>[2x]MGHHHHHHMGQLRLAVITTAKYFIPRLIGPFCQRYPGINVSLKVTNHEGLI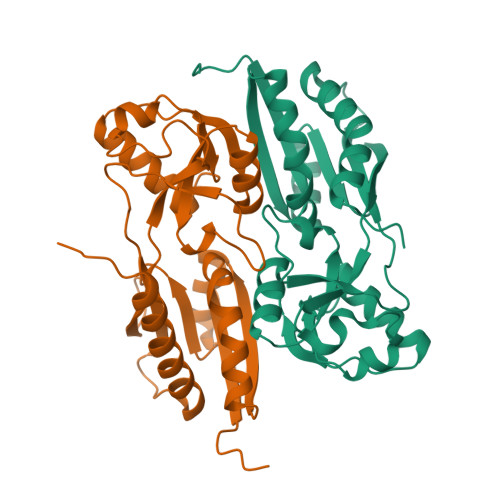NRINDNLDDLYVLSRPPSGFDITVQPFLDNPLVVVGPASHPLANQRGISLERLAQEPFILRERGSGTREATEQLFAAHNLNLNVKLDLGSNEAIKQAILGGLGLAVLSYHTLTSAGATPELKMFEVEGFPIHRQWHAVYPAGKQLSTVAATFLDYLLTESQRIAADIQIPESTTTDPELDAPQPVVGV> QYSSNTQQGRTSIVHLFEWRWVDIALECERYLAPKGFGGVQVSPPNENVAIHNPFRPWWERYQPVSYKLCTRSGNEDEFRNMVTRCNNVGVRIYVDAVINHMCGNAVSAGTSSTCGSYFNPGSRDFPAVPYSGADFNDGKCKTGSGDIENYNDATQVRDCRLSGLLDLALGKDYVRSKIAEYMNHLIDIGVAGFRIDASKHMAPGDIKAILDKLHNLNSNWFPEGSKPFIYQEVIDLGGEPIKSSDYFGNGRVTEFKYGAKLGTVIRKWNGEKMSALKNWGEGAGFMPSDRALVFVDNHDNQRGHGAGGASILTFADARLYKMAVGFMLAHPYGFTRVMSSYRWPRYFENGKDVNDWVGPPNDNGVTKEVTINPDTTCGNDWVCEHRARQIRNMVNFRNVVDGQPFTNWYDNGSNQVAFGRGNRGFIVFNNDDWTFSLTLQTGLPAGTYCDVISGDKINGNCTGIKIYVSDDGKAHF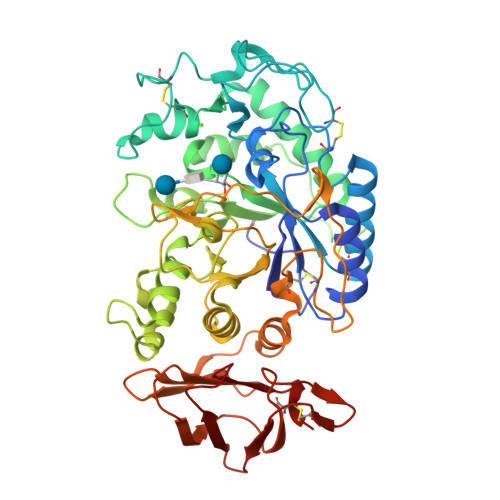SISNSAEDPFIAIHAESKL>MDNNKAEADTSSSMADPETRPTYTTHHLAIPSGVTQDEFDELKQSVVEFHTYQLSQNQCSSLLAQRIRAPNDVVWSIVRRFDQPQTYKHFIKSCSVSDNFTMAVGSTRDVNVISGLPAATSTERLDILDDDRQVTGFSIIGGEHRLRNYRSVT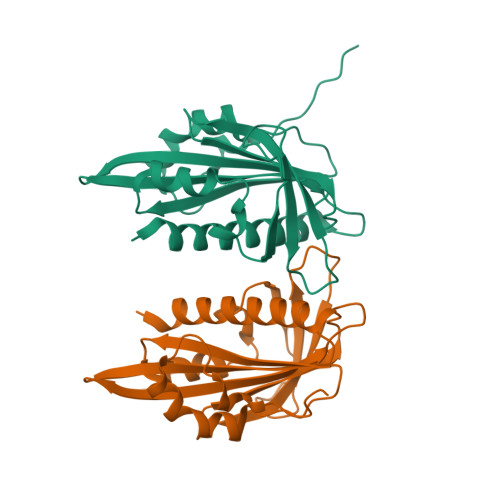SVHGFNRDGAICTVVLESYVVDVPEGNTEEDTRLFADTVVKLNLQKLVSVAESQVI[2x]> MHHHHHHGENLYFQGSSPSLEQDDGDEETSVVIVGKISFCPKDVLGHGAEGTIVYRGMFDNRDVAVKRILPECFSFADREVQLLRESDEHPNVIRYFCTEKDRQFQYIAIELCAATLQEYVEQKDFAHLGLEPITLLQQTTSGLAHLHSLNIVHRNLKPHNILISMPNAHGKIKAMISDFGLCKKLAVGRH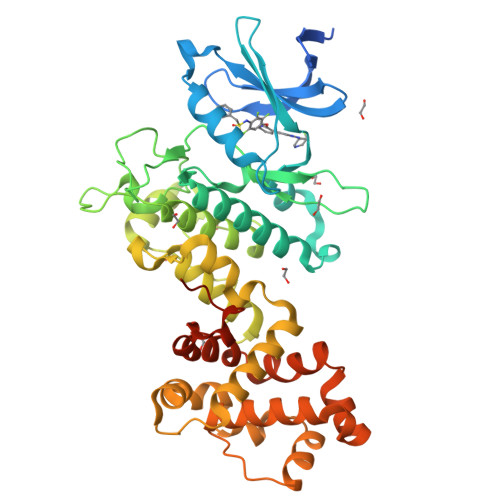SFSRRSGVPGTEGWIAPEMLSEDCKENPTYTVDIFSAGCVFYYVISEGSHPFGKSLQRQANILLGACSLDCLHPEKHEDVIARELIEKMIAMDPQKRPSAKHVLKHPFFWSLEKQLQFFQDVSDRIEKESLDGPIVKQLERGGRAVVKMDWRENITVPLQTDLRKFRTYKGGSVRDLLRAMRNKKHHYRELPAEVRETLGSLPDDFVCYFTSRFPHLLAHTYRAMELCSHERLFQPYYFHEPPEPQPPVTPDALGNS>MPPHGELQYLGQIQHILRCGVRKDDRTGTGTLSVFGMQARYSLRDEFPLLTTKRVFWKGVLEELLWFIKGSTNAKELSSKGVKIWDANGSRDFLDSLGFSTREEGDLGPVYGFQWRHFGAEYRDMESDYSGQGVDQLQRVIDTIKTNPDDRRIIMCAWNPRDLPLMALPPCHALCQFYVVNSELSCQLYQRSGDMGLGVPFNIASYALLTYMIAHITGLKPGDFIHTLGDAHIYLNHIEPLKIQLQREPRPFPKLRILRKVEKIDDFKAEDFQIEGYNPHPTIKMEMAV[6x]

TS is a pivotal enzyme in production of thymidine monophosphate and a well validated cancer target. Inhibition of TS leads to thymineless death characterized by DNA-damage, chromosomal fragmentation and concomitant induction of apoptosis. Novel classes of TS inhibitors with improved efficacy and resistance profiles could provide important complements to current TS directed drugs, for which there are reports of resistance. Here, we show for the first time that a CETSA-based screen for direct physical target engagement constitutes an attractive high throughput screening (HTS) strategy, which allows for the detection of known and novel TS inhibitors with cellular activity.

We investigated one of these, CBK115334 or 3-amino-2-benzoyl-4-methylthieno(2,3-b)pyridin-6-ol, which was chemically distinct from known TS inhibitors. Confirmatory data were obtained using CETSA on K562 cell lysates, which demonstrated a 3.7 °C shift at 200 μM. When applied to isolated recombinant human TS, 1 showed a 2.6 °C shift at 25 μM and a 5.2 °C shift at 100 μM and confirmed binding in the low μM range using surface plasmon resonance. We tested whether binding affected enzymatic activity of TS in vitro and observed 60% inhibition at 10 μM concentration and near complete inhibition at 100 μM. A crystal structure of TS with 1 revealed that the compound binds the active site of TS occupying the folate-binding pocket. The binding involves π–π stacking interactions with the substrate dUMP and polar interactions with residues lining the catalytic cavity (Asn112 and Arg50 in particular). This constitutes a novel mode of binding as compared with other anti-folates occupying this space. Amongst the new hits was 1, a μM inhibitor of the purified enzyme with sufficient cell penetration to result in intracellular target engagement and anti-proliferative effects in the high μM range. The binding mode of 1 to TS is partly new and it thus provides a potential starting point for further chemistry optimization.> AGRFTKVAAAVADSVVTIESVSDQEGMQGSGVIVDGRGYIVTNNHVISEAANNPSQFKTTVVFNDGKEVPANLVGRDPKTDLAVLKVDNVDNLTVARLGDSSKVRVGDEVLAVGAPLGLRSTVTQGIVSALHRPVPLSGEGSDTDTVIDAIQTDASINHGNSGGPLIDMDAQVIGINTAGKALSDSASGLGFAIPVNEMKLVANSLIKDGKIVHPTLGISTRSVSNAIASGAQVANVKAGSPAQ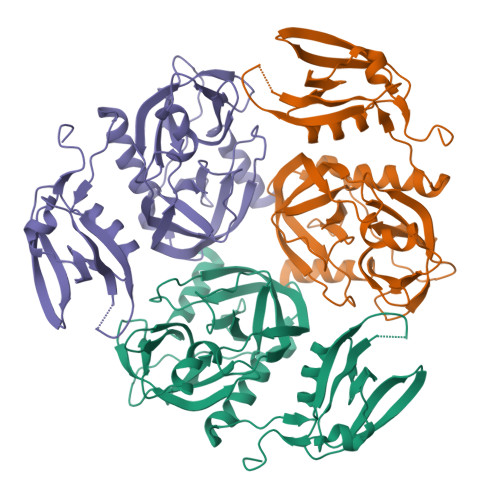KGGILENDVIVKVGNRAVADSDEFVVAVRQLAIGQDAPIEVVREGRHVTLTVKPDPDSTLEH> MHHHHHHGGSHHWGGDPARPALGVLELKSYALGVAVADAALRAAPVELLKCEPVEPGKALIMIRGEPEAVARAMAAALETAKAGSGNLIDHA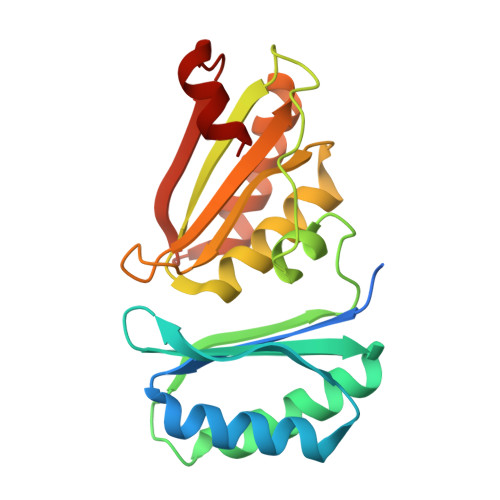FIGRIHPALLPFLLEETAAPPIEDPDEAVLVVETKTVAAAIEAADAALDVAPVRLLRMRLSEHIGGKAYFVLAGDEEAVRKAARAVRAVAGEKLIDLRIIPRPHEALRGRLFF>MDKTVKLWNRNGQLLQTLTGHSSSVTGVAFSPDGQTIASASDDKTVKLWNRNGQLLQTLTGHSSSVTGVAFSPDGQTIASASDDKTVKLWNRNGQLLQTLTGHSSSVTGVAFSPDGQTIASASDDKTVKLWNRNGQLLQTLTGHSSSVTGVAFSPDGQTIASASDDKTVKLWNRNGQLLQTLTGHSSSVTGVAFSPDGQTIASASDDKTVKLWNRNGQLLQTLTGHSSSVTGVAFSPDGQTIASASDDKTVKLWNRNGQLLQTLTGHSSSVTGVAFSPDGQTIASASD[4x]

β-Propeller proteins are common natural disc-like pseudo-symmetric proteins that contain multiple repeats (‘blades’) each consisting of a 4-stranded anti-parallel β-sheet. In the larger propellers a so-called “Velcro closure” is found, in which the N- and C-terminal β-strands are part of the same β-sheet, keeping the propeller closed. This “Velcro” can occur in different positions; in the “Velcro 1-3” variant, the closing β-sheet consists of one N-terminal and three C-terminal strands, while for the “Velcro 3-1” variant, the opposite is true. Starting from a highly repetitive β-propeller sequence, we designed a consensus motif sequence that formed a perfectly symmetric 7-bladed β-propeller.

To avoid bad interactions between the close termini, the N-terminal residue was removed. We decided to position the termini so that a glycine residue would be removed, theorizing this residues contribute little to the overall interaction energy and stability of the fold. In the case of V22WRAP-T, this was impossible as the loop lacks a glycine. Hence the central aspartate was removed instead. While the space group and packing differ between the crystals, the structure is identical for each protein. The crystal structures also show that the proteins are highly internally symmetric with a backbone RMSD between individual repeats below 0.3 Å. As expected, v22WRAP-T is the least stable protein, reflecting the fact this conformation is almost never seen in nature. In both Pizza and WRAP-T, the “Velcro 2-2” conformation is the least stabilising, which presumably explains why it is rarely observed in nature.> ARTMQT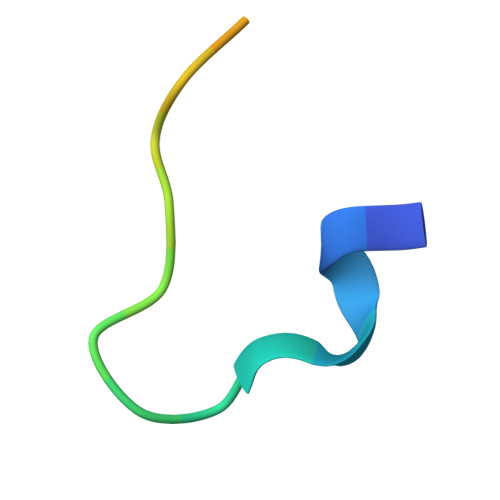ARKSTGGKAPRKQL> MAMSFEWPWQYRFPPFFTLQPNVDTRQKQLAAWCSLVLSFCRLHKQSSMTVMEAQESPLFNNVKLQR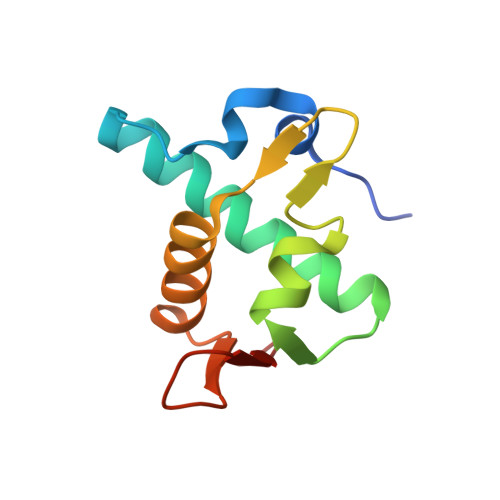KLPVESIQIVLEELRKKGNLEWLDKSKSSFLIMWR>[4x]SMNFYSAYQHGFVRVAACTHHTTIGDPAANAASVLDMARACHDDGAALAVFPELTL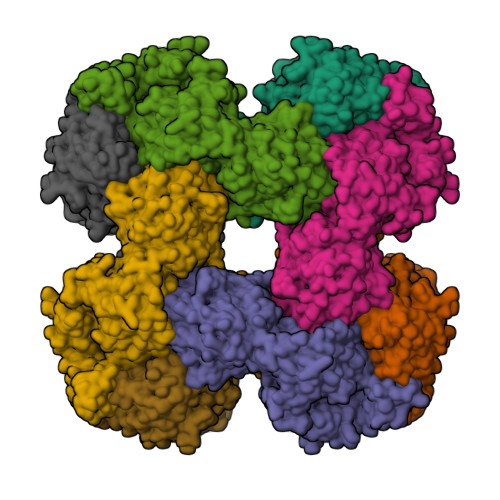SGYSIEDVLLQDSLLDAVEDALLDLVTESADLLPVLVVGAPLRHRHRIYNTAVVIHRGAVLGVVPKSYLPTYREFYERRQMAPGDGERGTIRIGGADVAFGTDLLFAASDLPGFVLHVEIAEDMFVPMPPSAEAALAGATVLANLSGSPITIGRAEDRRLLARSASARCLAAYVYAAAGEGESTTDLAWDGQTMIWENGALLAESERFPKGVRRSVADVDTELLRSERLRMGTFDDNRRHHRELTESFRRIDFALDPPAGDIGLLREVERFPFVPADPQRLQQDCYEAYNIQVSGLEQRLRALDYPKVVIGVSGGLDSTHALIVATHAMDREGRPRSDILAFALPGFATGEHTKNNAIKLARALGVTFSEIDIGDTARLMLHTIGHPYSVGEKVYDVTFENVQAGLRTDYLFRIANQRGGIVLGTGDLSELALGWSTYGVGDQMSHYNVNAGVPKTLIQHLIRWVISAGEFGEKVGEVLQSVLDTEITPELIPTGEEELQSSEAKVGPFALQDFSLFQVLRYGFRPSKIAFLAWHAWNDAERGNWPPGFPKSERPSYSLAEIRHWLQIFVQRFYSFSQFKRSALPNGPKVSHGGALSPRGDWRAPSDMSARIWLDQIDREVPKG Specifically, the β-­glycosidic bond of 6′-P-β-glucoside is cleaved by 6-P-β-glucosidase (6PβGlu; EC 3.2.1.86), releasing 6-P-β-glucose (BG6; glycon), an important cellular precursor, and the remaining portion of the given substrate (aglycon). Here, the high-resolution crystal structures of GH1 6-P-β-glucosidases from Lactobacillus plantarum (LpPbg1) and Streptococcus mutans (SmBgl) and their complexes with ligands are reported. 6PβGlu is a single-domain protein that adopts a (β/α)8-barrel (TIM-barrel) structure, which is a typical fold of GH1-family members. The GH1-family enzymes utilize a double-displacement mechanism of catalysis with retention of configuration at the anomeric C atom of the glycon moiety.

SmBgl was also crystallized in the presence of the reaction product 6-P-β-glucose. SmBgl–BG6 crystallized in the monoclinic space group P21 with two protein molecules in the asymmetric unit. The final model consisted of residues Ala0–Ile477 in both chains as well as 1145 water molecules, five ethylene glycol molecules, two formate ions and two BG6 ligands. Substrate-bound and product-bound complexes of SmBgl contain a phosphoryl group attached to the glucose ring occupying the phosphate-dedicated cavity. The O3 and O4 hydroxyl groups are both kept in place by Gln18 and, in the case of O3, also by His130. The position of the β-­glucose O6 atom nearly corresponds to the glycosidic O atom of PSC and the O1 atom of BG6.

>[2x]SNAMSKLPENFLWGGAVAAHQLEGGWQEGGKGISVADVMTAGRHGVAREITAGVLEGKYYPNHEAIDFYHHYKEDVKLFAEMGFKCFRTSIAWTRIFPKGDEAEPNEAGLQFYDDLFDECLKYGIEPVVTLSHFELPYHLVTEYGGFTNRKVIDFFVHFAEVCFRRYKDKVKYWMTFNEINNQANYQEDFAPFTNSGIVYKEGDDREAIMYQAAHYELVASARAVKIGHAINPNLNIGCMVAMCPIYPATCNPKDILMAQKAMQKRYYFADVHVHGFYPEHIFKYWERKAIKVDFTERDKKDLFEGTVDYIGFSYYMSFVIDAHRENNPYYDYLETEDLVKNPYVKASDWDWQIDPQGLRYALNWFTDMYHLPLFIVENGFGAIDQVEADGMVHDDYRIDYLGAHIKEMIKAVDEDGVELMGYTPWGCIDLVSAGTGEMRKRYGFIYVDKDDEGKGTLKRSPKLSFNWYKEVIASNGDDI>[2x]GSMAPRAGFDAEQVRDKARKDLLHLLEGVRGKKNLVIEKDLAGPLGVIVKASTLRDYGVDNFFFLENKNTGTSQRNIVFIARGESVRNAHAIAAQIKRIQRESQTSHDFHIFWVPRRTLFSDKVLEEAGVLGDANISELPLYFFPLERDVLSLELNDSFR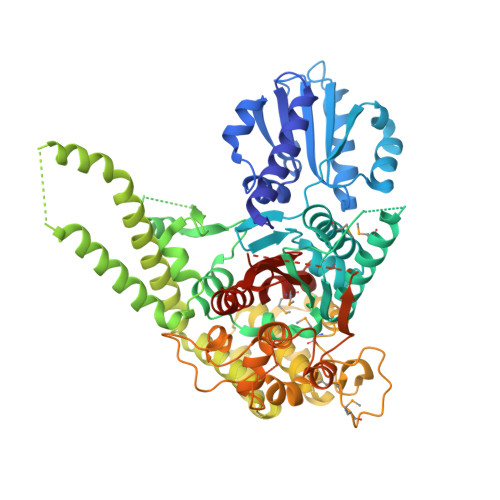DLYLAKDPTPVFLLSRALMGIQKKHGLFPRIIGKGENAKRVADLLSRMRQELLAGEEAGESDRAGLSPSTTIESVIIIDREVDFVTPLLTQLTYEGLIDEYFGIQNNQTDVDAVIVGAPAQSAASTSTAVPTNSSQSRKRKIQLDGSDSLYSQLRDANFAIVGSLLNTVARRLKSDYESRHNTKTTAELKEFVKKLPGYQAEQQSLKIHSNIAEEIINYTRTEIFNKLLEVQQNLAAGADPSSQFDSIEELVARDTPLPQVLRLLCLYSCISGGIKTKELDHFRRLVLQGYGHQHLLTLHNLERLQMFLSKSSPLASMITMSGSSGGPDQKTNYTYLRKQLRLIVDEVNEQDPNDIAYVYSGYAPLSIRLVQCVLQKQYLLSITKGSGTVIAAGPVAGGGAQGWKGFEEIVKHARGPTFDEIQKGEDKAVKARALLSGSSGDKKTVFVVFVGGITFTEIAALRFIAKQEEARRNIVICTTSIINGNRMMNAAIETATFEKTTVTTAAAQ> MTKKVGLLVMAYGTPYKDEDIERYYTDIRHGHKPSEEMIADLRGRYHAIGGLSPLAKITEAQAYGLEKALNDSQDEVEFKAYIGLKHIEPFIEDAVEAMHKDGIEEAISIVLAPHYSSFSVEAYNKRAKEAADKLGGPRINAINDWYKQPKFIQMWADRINETAKQIPADELLDTVLIVSAHSLPEKIKQHNDPYPNQLQETADFIFEKVVVPHYALGWQSEGKTGEPWLGPDVQDLTRELYGREKYKHFIYTPVGFVAEHLEVLYDNDYECKVVTDEVGAAYHRPPMPNSDPEFLEVLRTVVWEKYSNL

Coproporphyrin ferrochelatase (CpfC) in the CPD heme biosynthesis pathway incorporates ferrous iron into coproporphyrin III (cpIII) to give coproheme, which is eventually decarboxylated to yield heme b by the coproheme decarboxylase enzyme in the final step of this biosynthetic process (Dailey et al., 2017; Dailey & Gerdes, 2015; Layer, 2021). Understanding structure–function relationships of key enzymes, such as ferrochelatase, is an essential precondition for the design of new inhibitors for antibiotic‐resistant pathogens, like Listeria monocytogenes. LmCpfC crystals in complex with cpIII were soaked with a ferrous iron solution and flash‐vitrified after 2, 3, and 4 min, to obtain snapshots of the enzymatic reaction during iron insertion into the porphyrin macrocycle. We report three crystal structures showing different iron content during metalation in LmCpfC, identifying the presence and defining the extent of the porphyrin distortions during iron insertion.

In the “34% Fe” structure (resolution 2.15 Å) best statistics were obtained with a 34% iron occupancy fitted into the electron density, which is located slightly toward pyrrole ring C and D and now in plane with the substrate. Ring A with the substituent p2 exhibits the highest distortion in the “34% Fe” structure (+12.6°), +9.2° in the cpIII structure and lowered values for the “24% Fe” (+4.8°), and the “68% Fe” (+1.9°) structures; in ring B (p4) the angle is altered the most in the analyzed samples (−13.4°, −10.5°, −11.4°, and −6.7°) as a function of the site occupancy by Fe ions, exhibiting a high degree of distortion compared to the coproheme structure. Since its activation is an indication of a saddling (B2u) deformation, these data suggest the formation of a stable intermediate species, consisting of a distorted porphyrin macrocycle in equilibrium with the substrate (cpIII) and the product (coproheme). These data agree with the observed structures representing fractions of iron in cpIII of "24% Fe", "34% Fe", and "68% Fe", where the structure between 0.3 and 0.4 eq of the metal shows the largest porphyrin distortion. The metalation mechanism includes a porphyrin saddling distortion, which becomes predominant both in the crystal and in solution at iron to cpIII ratios between 0.3 and 0.4. The measured change of angles throughout the ferrous iron insertion process at the site of p7 at pyrrole ring D is also peculiar: the rings in the substrate‐ and product‐bound states overlap well for all structures besides the “24% Fe” structure (−2.1° in the cpIII‐structure, −1.6° in the "68% Fe" structure, and −1.4° in the "34% Fe" structure). The residue points toward p7 in the “24% Fe”, “34% Fe”, and in the coproheme‐complex structures, but points away (5.4 Å) in the “68% Fe” structure.> GPAAMSGSIPEIYLDVVTKETISDKYKDWHFISKN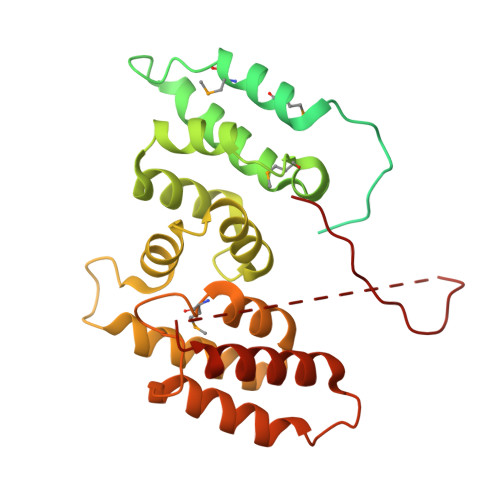CHYEQLMDLEMKDTAYSFLFGSSRSQGKVPEFVHLKCPSITNLLVLFGVNQEKCNSLKINYEKKENSRYDNLCTIFPVNKMLKFLMYFYSDDDNDDVREFFLKAFICLILDRKVFNAMESDHRLCFKVLELFNEAHFINSYFEIVDKNDFFLHYRLLQIFPHLQSALLRRRFSEKQGRTETIQQNIIKEFNEFFDCKNYKNLLYFILTMYGSKFIPFGPKCQVTEYFKDCILDISNETTNDVEISILKGILNLFSKIRGXXXXXXXXXXXXXX> ASTTGG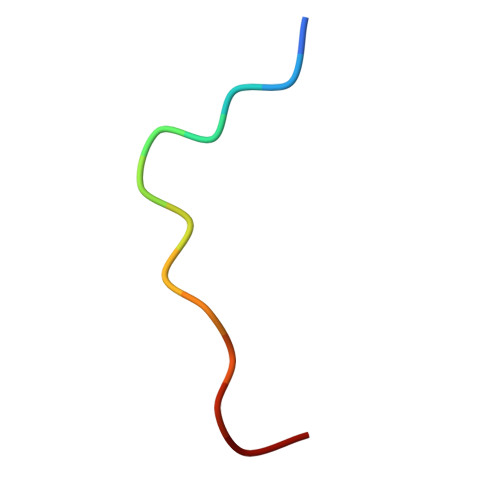NSQRGSG>[2x]ALYEDPPDQKTSPSGKPATLKICSWNVDGLRAWIKKKGLDWVKEEAPDILCLQETKCSENKLPAELQELPGLSHQYWSAPSDKEGYSGVGLLSRQAPLKVSYGIGDEEHDQEGRVIVAEFDSFVLVTAYVPNAGRGLVRLEYRQRWDEAFRKFLKGLASRKPLVLCGDLNVAHEEIDLRNPKGNKKNAGFTPQERQGFGELLQAVPLADSFRHLYPNTPYAYTAWTYMMNARSKNVGWRLDYFLLSHSLLPALCDSKIRSKALGSDHCPITLYLAL

The BER pathway is comprised of several factors; the scaffolding protein XRCC1, a damage-specific DNA glycosylase to remove the damaged base, apurinic/apyrimidinic endonuclease (APE1) to cleave the DNA backbone 5′ of the resulting apurinic/apyrimidinic (AP) site, DNA polymerase (pol) β to synthesize the DNA, and DNA ligase III to seal the repaired DNA. Two predominant APE1 DNA cleavage reactions are (1) AP-endonuclease (AP-endo) and (2) exonuclease (exo). APE1 exo activity removes 3′ end groups, including oxidatively damaged DNA bases, chain terminating nucleotide analog drugs, terminal blocking groups, and mismatched bases. Our structures demonstrate APE1 uses the same active site to exonucleically remove 3′ mismatches and DNA damage by a non-base flipping mechanism.

Our structures indicate that the side chains of both W280 and F266 reduce the size of the APE1 active site, and previous steady-state kinetic analyses indicate W280A and F266A APE1 mutants increase the exo catalytic rate. The F266A APE1 mutation had the most dramatic effect on exo activity, with a ~20-fold increase in the observed burst rate and a ~50-fold increase in the steady-state rate at 21 ± 7 s−1 and 2.1 ± 0.7 s−1, respectively. Notably, this burst rate is close to what we observed for the APE1 AP-endo reaction (<2-fold difference) and the steady-state rate exceeds that observed for the AP-endo reaction by ~threefold. To further elucidate the catalytic role of F266 in the exo reaction, we obtained a 2.0 Å substrate complex structure of F266A APE1 bound to DNA containing a C/T mismatch at the 3′ end of a nick and a PS linkage modification 5′ to the C. The structure revealed that mutating F266 to an alanine expands the size of the APE1 active site, allowing the mismatched C to occupy an alternate conformation. When the mismatched C and F266 in the WT-APE1 structure are overlaid with those in the F266A APE1 structure, it is revealed that the mismatched C has rotated by ~120° in the mutant structure into a part of the active site that is normally occupied by the F266 side chain. Our kinetics show that rates for both the chemistry step and the product release step of the exo reaction on a mismatch are reduced in comparison to the AP-endo reaction by only ~40-fold and ~18-fold, respectively. This reduction in rate is recovered by the single F266A mutation, which increases space in the APE1 active site and allows the mismatched base to adopt an alternative conformation. A restrictive active site and larger exo substrate may be responsible for the reduced incision rate for the APE1 exo reaction.>MSLQRIVRVSLEHPTSAVCVAGVETLVDIYGSVPEGTEMFEVYGTPGVDIYISPNMERGRERADTRRWRFDATLEIIVVMNSPSNDLNDSHVQISYHSSHEPLPLAYAVLYLTCVDISLDCDLNCEGRQDRNFVDKRQWVWGPSGYGGILLVNCDRDDPSCDVQDNCDQHVHCLQDLEDMSVMVLRTQGPAALFDDHKLVLHTSSYDAKRAQVFHICGPEDVCEAYRHVLGQDKVSYEVPRLHGDEERFFVEGLSFPDAGFTGLISFHVTLLDDSNEDFSASPIFTDTVVFRVAPWIMTPSTLPPLEVYVCRVRNNTCFVDAVAELARKAGCKLTICPQAENRNDRWIQDEMELGYVQAPHKTLPVVFD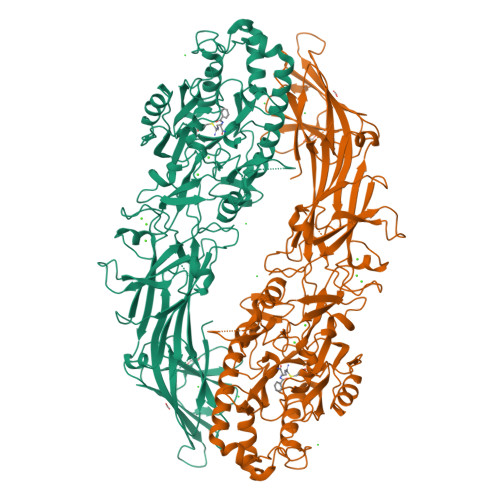SPRNGELQDFPYKRILGPDFGYVTREPRDRSVSGLDSFGNLEVSPPVVANGKEYPLGRILIGGNLPGSSGRRVTQVVRDFLHAQKVQPPVELFVDWLAVGHVDEFLSFVPAPDGKGFRMLLASPGACFKLFQEKQKCGHGRALLFQGVVDDEQVKTISINQVLSNKDLINYNKFVQSCIDWNREVLKRELGLAECDIIDIPQLFKTERKKATAFFPDLVNMLVLGKHLGIPKPFGPIINGCCCLEEKVRSLLEPLGLHCTFIDDFTPYHMLHGEVHCGTNVCRKPFSFKWWNMVP[3x]>[6x]LDKVYQMKSKPRGYCLIINNHNFAKAREKVPKLHSIRDRNG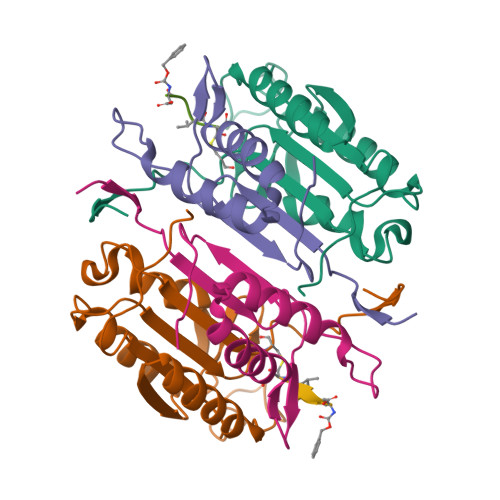THLDAGALTTTFEELHFEIKPHHDCTVEQIYEILKIYQLMDHSNMDCFICCILSHGDKGIIYGTDGQEAPIYELTSQFTGLKCPSLAGKPKVFFIQACQGDNYQKGIPVETD;>TRYIPDEADFLLGMATVNNCVSYRNPAEGTWYIQSLCQSLRERCPRGDDILTILTEVNYEVSNKDDKKNMGKQMPQPTFTLRKKLVFPS[6x];>XDEVD[6x]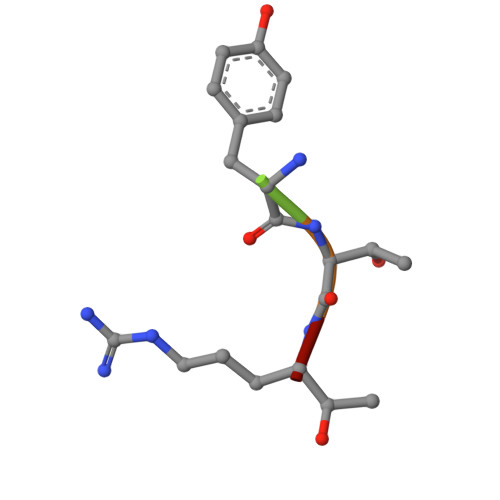> WYTRX>[2x]MEGMLKGEGPGPLPPLLQQYVELRDQYPDYLLLFQVGDFYECFGEDAERLARALGLVLTHKTSKDFTTPMAGIPLRAFEAYAERLLKMGFRLAVADQVEPAEEAEGLVRREVTQLLTPGTLLQESLLPREANYLAAIATGDGWGLAFLDVSTGEFKGTVLKSKSALYDELFRHRPAEVLLAPELLENGAFLDEFRKRFPVMLSEAPFEPEGEGPLALRRARGALLAYAQRTQGGALSLQPFRFYDPGAFMRLPEATLRALEVFEPLRGQDTLFSVLDETRTAPGRRLLQSWLRHPLLDRGPLEARLDRVEGFVREGALREGVRRLLYRLADLERLATRLELGRASPKDLGALRRSLQILPELRALLGEEVGLPDLSPLKEELEAALVEDPPLKVSEGGLIREGYDPDLDALRAAHREGVAYFLELEERERERTGIPTLKVGYNAVFGYYLEVTRPYY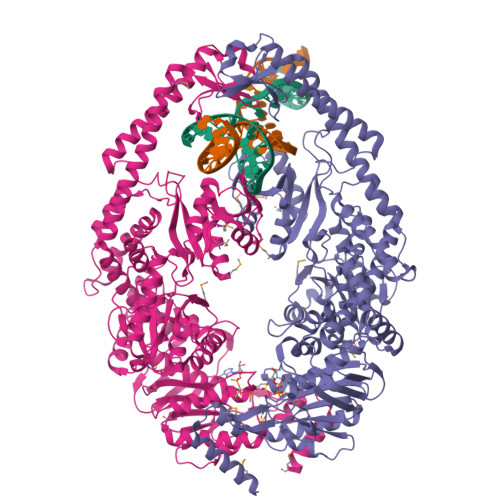ERVPKEYRPVQTLKDRQRYTLPEMKEKEREVYRLEALIRRREEEVFLEVRERAKRQAEALREAARILAELDVYAALAEVAVRYGYVRPRFGDRLQIRAGRHPVVERRTEFVPNDLEMAHELVLITGPNMAGKSTFLRQTALIALLAQVGSFVPAEEAHLPLFDGIYTRIGASDDLAGGKSTFMVEMEEVALILKEATENSLVLLDEVGRGTSSLDGVAIATAVAEALHERRAYTLFATHYFELTALGLPRLKNLHVAAREEAGGLVFYHQVLPGPASKSYGVEVAAMAGLPKEVVARARALLQAMAARREG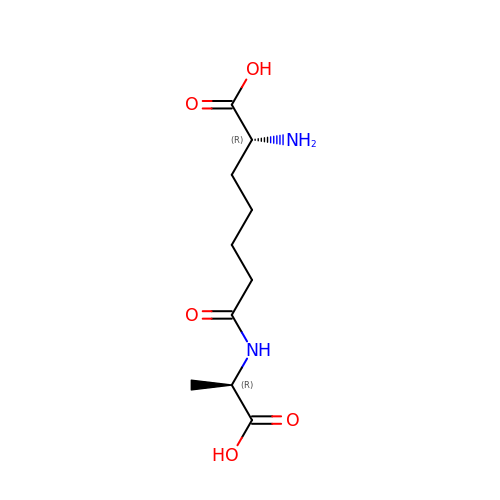(2R)-2-AMINO-7-{[(1R)-1-CARBOXYETHYL]AMINO}-7-OXOHEPTANOIC ACID | C10 H18 N2 O5 | GMHVWLJCMCGBKZ-RNFRBKRXSA-N>GPSPNYDKWEMERTDITMKHKLGGGQYGEVYEGVWKKYSLTVAVKTLKEDTMEVEEFLKEAAVM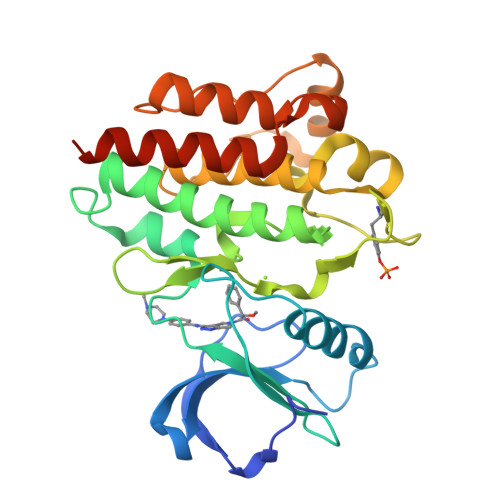KEIKHPNLVQLLGVCTREPPFYIIIEFMTYGNLLDYLRECNRQEVNAVVLLYMATQISSAMEYLEKKNFIHRDLAARNCLVGENHLVKVADFGLSRLMTGDTYTAHAGAKFPIKWTAPESLAYNKFSIKSDVWAFGVLLWEIATYGMSPYPGIDLSQVYELLEKDYRMERPEGCPEKVYELMRACWQWNPSDRPSFAEIHQAFETMFQESSISDEVEKELGK[2x]DC-SIGN (dendritic-cell-specific intercellular adhesion molecule 1-grabbing nonintegrin; CD209) and DC-SIGNR (DC-SIGN-related receptor, also known as L-SIGN and variously designated CD209L and CD299) are glycan-binding receptors of the immune system. DC-SIGN is expressed on dendritic cells and some types of macrophages, while DC-SIGNR is expressed on sinusoidal endothelial cells and in the placenta. Although each of these receptors binds mannose and related monosaccharides, they have differing specificities for oligosaccharides and for surfaces of microorganisms. Both DC-SIGN and DC-SIGNR bind high mannose oligosaccharides found on viral envelope glycoproteins and can participate in viral infection either directly by facilitating viral entry into a target cell or indirectly by presenting viruses to target cells. The CRDs in DC-SIGN and DC-SIGNR tetramers are projected at the ends of extended neck regions formed from a series of conserved but not identical sequences of 23 amino acids.

Further truncated forms were generated by removing the N-terminal non-repeat region or by removing this region and the first half of the first repeat unit. Gel filtration suggested that the purified truncated fragment is tetrameric, and differential scanning calorimetry demonstrated that it retains the stability of the full-length DC-SIGNR neck region, with a melting temperature of 81.7 °C compared with the measured value of 80.1 °C for the full-length neck. The structure was determined by multiwavelength anomalous dispersion phasing using crystals soaked in Pb(CH3COO)2. Within the unit cell, four molecules interact around the crystallographic 4-fold axis to generate a four-helix bundle. The four-helix bundles are translated by various numbers of repeats along the c axis throughout the crystal. This arrangement produces a unit cell with an asymmetric unit one repeat long that is an average of six nearly identical repeats. The model was further refined in Phenix to 2.2 Å. Completely conserved residues were given occupancy of 1.0, and side chains at the non-conserved positions were built with occupancy assigned based on their frequency in repeats 2 through 7: proline with occupancy of 0.83 and serine with occupancy of 0.17 at position 1 as well as glutamate with occupancy of 0.17, glutamine with occupancy of 0.33, and arginine with occupancy of 0.5 at position 15, resulting in the final refined model described in Table 2. The structure of the neck unit representing repeats 2 through 7 of the neck of DC-SIGNR is predominantly that of a four-helix bundle. The sequence of amino acids in the helical portions of the repeats follows the expected heptad pattern, with hydrophobic amino acids at the a and d positions. These hydrophobic residues are positioned toward the center of the bundle and pack against one another.

> GELPEKSKLQEIYQELTRLKAAVGELPEKSKLQEIYQELTRLKAAVGELPEKSKLQEIYQELTRLKAAVGELPEKSKLQEIYQELTRLKAAVGELPEKSKLQEIYQELTELKAAVGELPEKSKLQEIYQELTQLKAAVGELPDQSKQQQIYQELTDLKTAFERLGHH>[2x]MKIQHIIHENQLGLLFQQGSFGLEKESQRVTADGAIVTTPHPAVFGNRRYHPYIQTDFAESQLELITPPTKKLEDTFRWLSVIHEVVQRSLPEEEYIFPLSMPAGLPAEEQIRVAQLDNPEDVAYREYLVKIYGKNKQMVSGIHYNFQLSPDLITRLFRLQNEYQSAVDFQNDLYLKMAKNFLRYQWILLYLLAATPTVESAYFKDGSPLAKGQFVRSLRSSQYGYVNDPEINVSFDSVEKYVESLEHWVSTGKLIAEKEFYSNVRLRGAKKAREFLTTGIQY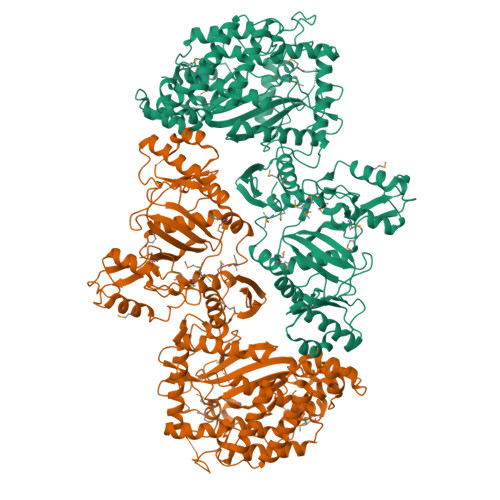LEFRLFDLNPFEIYGISLKDAKFIHVFALFMIWMDHTADQEEVELGKARLAEVAFEHPLEKTAYAVEGELVLLELLSMLEQIGAEPELFEIVKEKLTQFTDPSKTVAGRLVRAIEQAGSDQQLGAQLAQQYKAQAFERFYALSAFDNMELSTQALLFDVIQKGIHTEILDENDQFLCLKYGDHIEYVKNGNMTSHDSYISPLIMENKVVTKKVLQKAGFNVPQSVEFTSLEKAVASYALFENRAVVIKPKSTNYGLGITIFQQGVQNREDFAKALEIAFREDKEVMVEDYLVGTEYRFFVLGDETLAVLLRVPANVVGDSVHSVAELVAMKNDHPLRGDGSRTPLKKIALGEIEQLQLKEQGLTIDSIPAKDQLVQLRANSNISTGGDSIDMTDEMHESYKQLAVGITKAMGAAVCGVDLIIPDLKQPATPNLTSWGVIEANFNPMMMMHIFPYAGKSRRLTQNVIKMLFPELE A novel enteric T cell superantigen, I2, and its full-length gene product pfiT, are encoded by a microbial gene associated with Crohn's disease (CD). Crystal structure of pfiT at high resolution revealed that pfiT belongs to the bacterial transcription factor family of tetracycline repressor (TetR). We show that pfiT specifically and directly interacts with class II MHC HLA-DR, and to a lesser extent HLA-DP or HLA-DQ, and show that pfiT shares an overlapping binding site on HLA-DR1 with other superantigens. We show that pfiT can stimulate the activation of both mouse splenocytes and human peripheral blood mononuclear cells (PBMCs).

Based upon the high resolution crystal structure of pfiT, we found that pfiT belongs to the TetR transcription regulator protein family. The TetR family members are key players in multidrug resistance, virulence, and pathogenicity processes caused by bacterial pathogens. They act as repressors by binding to consecutive DNA major grooves through the N-terminal DBDs. TetR proteins function as a dimer to bind their DNA elements. Our results demonstrated that pfiT exists as a dimer in solution; and crystal structure also confirmed that pfiT is a dimer at structural level. An apparent molecular mass of 48 KDa was obtained with a local root-mean-square (rms) deviation of 0.007 OD and a global χ2 of 1.5, with molecular mass being the only fitting parameter. This value is in good agreement with the theoretically calculated mass of 45 KDa for a pfiT dimer, suggesting again that pfiT exists as a dimer in solution. Our structural study indicated that the structures of both pfiT and MAM are completely helical, although pfiT displays a different folding pattern. The distinct structure of pfiT relative to other SAgs suggests that it represents a novel family of SAg.

>GPLGSMRTMVDSGQLTDPESARGKLLQTAAHLFRNKGFERTTVRDLASAVGIQSGSIFHHFKSKDEILRAVMEETIHYNTAMMRASLEEASTVRERVLALIRCELQSIMGGSGEAMAVLVYEWRSLSAEGQAHVLALRDVYEQIWLQVLGEAKAAGYIRGDVFITRRFLTGALSWTTTWFRAQGSLTLEELAEEALLMVLKSD[2x]> MKQALRVAFGFLILWASVLHAEVRIVIDSGVDSGRPIGVVPFQWAGPGAAPEDIGGIVAADLRNSGKFNPLDRARLPQQPGSAQEVQPAAWSALGIDAVVVGQVTPNPDGSYNVAYQLVDTGGAPGTVLAQNSYKVNKQWLRYAGHTASDEVFEKLTGIKGAFRTRIAYVVQTNGGQFPYELRVSDYDGYNQFVVHRSPQPLMSPAWSPDGSKLAYVTFESGRSALVIQTLANGAVRQVASFPRHNGAPAFSPDGSKLAFALSKTGSLNLYVMDLASGQIRQVTDGRSNNTEPTWFPDSQNLAFTSDQAGRPQVYKVNINGGAPQRITWEGSQNQDADVSSDGKFMVMVSSNGGQQHIAKQDLATGGVQVLSSTFLDETPSLAPNGTMVIYSSSQGMGSVLNLVSTDGRFKARLPATDGQVKFPAWSPYLLEHHHHHH;> MPGFNYGGKGDG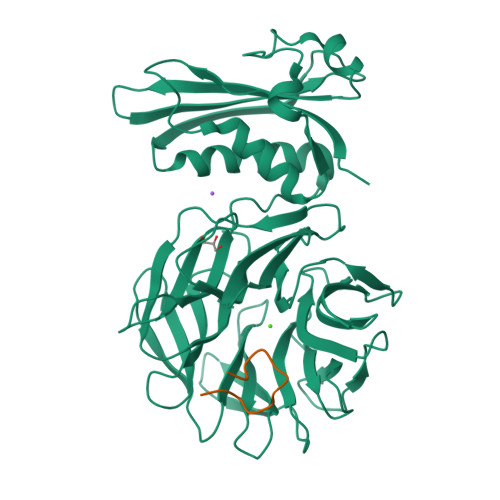TGWSSERGSGPEPGGGSHGNSGGHDRGDSSNVGNESVTVMKPGDSYNTPWGKVIINAAGQPTMNGTVMTADNSSMVPYGRGFTRVLNSLVNNPVSLEHHHHHH>[4x]GSHMDSTTIQQNKDTLSQIVVFPTGNYDKNEANAMVNRLANIDGKYLNALKQNNL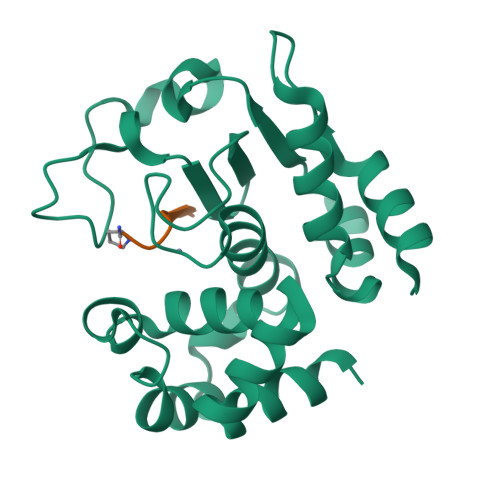KIKLLSGKLTDEKEYAYLKGVVPKGWEGTGKTWDDVPGLGGSTVALRIGFSNKGKGHDAINLELHATAHAIDHIVLNDISKSAQFKQIFAKEGRSLGNVNFLGVYPAEFFAESFAYYYLNQDTNSKLKSACPQTYSFLQNLAK;>[4x]XEVNAPVP>GSHMMEFKTDIEIAQEANPQDIRDIAKKINLSEDDIELYGKYKAKIDYNVLNRTKSRAGKLILTTAINPTPAGEGKTTTSIGVADALAKLGKNVIAALREPSMGPVFGIKGGAAGGGYAQVVPMEDINLHFTGDMHAIGAANNLLAAMLDNHVYQTNSLNINPKRITWRRCVDMNDRQLRNVVDGLGKKVDGVTREDGFDITVASEVMAAFCLSNNISELKENLGNIVVAYNYSGKPVTARDLNAHGAMAAILKDALKPNLVQTLEGTPAILHGGPFANIAHGCNSIIATKMGMHMADYVVTEAGFGADLGAEKFLDIKCRKAGIRPDAVIIVATVRALKYNGGVAKDQLNNENLEALEKGLPNLLKHIENITQVYKIPAVVAINRFPLDTDAELALVRSKCEELGVKVALSEVWANGGEGGIEVANEVLKLIEEGENNFEYCYEEDMTIKEKLNAIATKIYGADGVNYTKEANKQIAELEELGFGNLPVCVAKTQYSLSDDQTKLGRPTGFTIEVRQANISAGAGFVVVMTGEIMKMPGLPKLPAAERIDVDENGKISGLF[4x]

FtfL is a key enzyme in C1 metabolism pathway. It catalyzes the synthesis of formyltetrahydrofolic acid from formic acid and tetrahydrofolic acid. Formyltetrahydrofolic acid is then converted through two reactions to 5,10-methylene tetrahydrofolic acid, a metabolite for biosynthesis of pyrimidines and amino acids. PaFtfL exhibits a tetramer in all three crystal structures, consistent with other reported FtfL crystal structures.

To further investigate the structural mechanism of FtfL inhibition by BBR, we determined the crystal structures of PaFtfL apo enzyme, PaFtfL complexed with its substrate ATP, as well as PaFtfL complexed with BBR at 2.0 Å, 2.3 Å, and 2.6 Å resolutions, respectively. Structural comparison among our crystal structures of PaFtfL-BBR, PaFtfL-ATP, and MtFtfL-folate suggests that BBR overlaps with ATP and tetrahydrofolate on binding to FtfL, indicating that BBR likely competes with ATP and tetrahydrofolate to bind FtfL active site. Through structural analysis of PaFtfL-BBR complex, we revealed the interaction sites of FtfL, namely “active site” and “allosteric site. Comparison of the structures of enzyme–substrate complexes PaFtfL-ATP and MtFtfL-folic acid showed that the FtfL binding sites of both substrates significantly overlapped with the “active site” described above, suggesting that BBR may inhibit FtfL activity by competing with ATP and tetrahydrofolic acid for binding to this site. Each protomer comprises its own solvent-exposed active site close to the protomer interface. Structural comparison reveals that PaFtfL adopts essentially the same overall fold for each of the protomers and exhibits an identical active site as in reported crystal structures of FtfL from other bacterial species, indicative its conserved catalytic mechanism.> ATTTMTMIQALRSAMDVMLERDDNVV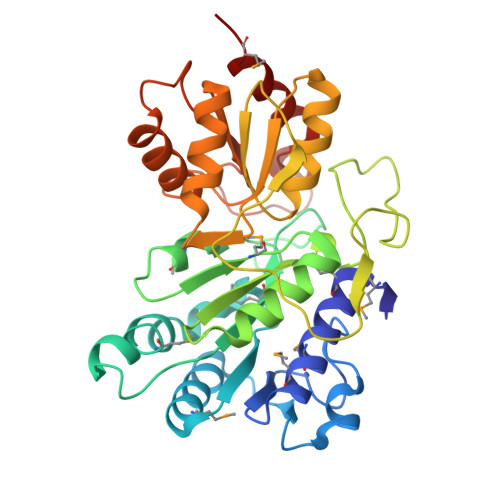VYGQDVGYFGGVFRCTEGLQTKYGKSRVFDAPISESGIVGTAVGMGAYGLRPVVEIQFADYFYPASDQIVSEMARLRYRSAGEFIAPLTLRMPCGGGIYGGQTHSQSPEAMFTQVCGLRTVMPSNPYDAKGLLIASIECDDPVIFLEPKRLYNGPFDGHHDRPVTPWSKHPHSAVPDGYYTVPLDKAAITRPGNDVSVLTYGTTVYVAQVAAEESGVDAEVIDLRSLWPLDLDTIVESVKKTGRCVVVHEATRTCGFGAELVSLVQEHCFHHLEAPIERVTGWDTPYPHAQEWAYFPGPSRVGAALKKVMEV4-[2-[4-(aminomethyl)phenyl]phenyl]piperazin-2-one | C17 H19 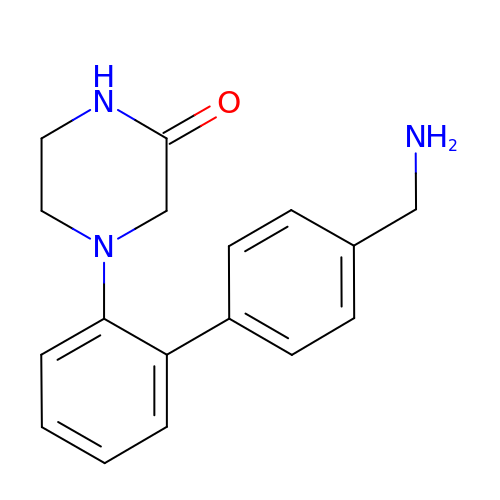N3 O | PENSDGIWXYUOBB-UHFFFAOYSA-N> KVYYLPVTLTQFQKDLSEILISLHAKSFKASIIGEPQADAVNKPSG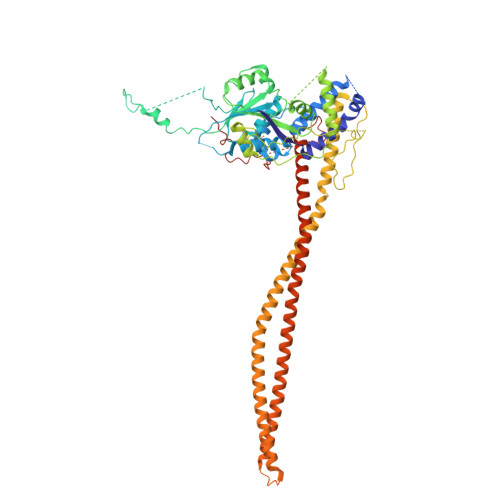LPAGPETHPYPTLSQRQLTYIFDSNIRAIANHPSLLVDHYMPRQLLRMEPTESSIAGSHKFQVLNQLINSICFRDREGSPNEVIKCAIIAHSIKELDLLEGLILGKKFRTKRLSGTSLYNEKHKFPNLPTVDSTINKDGTPNSVSSTSSNSNSTSYTGYSKDDYDYSVKRNLKKRKINTDDWLFLATTKHLKHDQYLLANYDIDMIISFDPMLEVELPALQVLRNNANKDIPIIKLLVQNSPDHYLLDSEIKNSSVKSSHLSNNGHVDDSQEYEEIKSSLLYFLQARNAPVNNCEIDYIKLVKCCLEGKDCNNILPVLDLITLDEASKDSSDSGFWQPQLTKLQYSSTELPLWDGPLDIKTYQTELMHRAVIRLRDIQDEYAKGTVPLYEKRLNETQRQNQLDEIKNSVGLTFKKKQEVEKSINDSEKRLKHAMTESTKLQNKINHLLKNRQELENFNKLPSNTISSENHLEEGSALADKLKEYIDKNATLFNKLKELQQANAEKSKLNDELRSKYQIESSKAAESAQTLKILQESMKSLENEVNGPLTKFSTESLKKELERLQNDFQSLKARNKFLKNYITL> MTADELVFFVNGKKVVEKNADPETTLLAYLRRKLGLRGTKLGCGEGGCGACTVMLSKYDRLQDKIIHFSANACL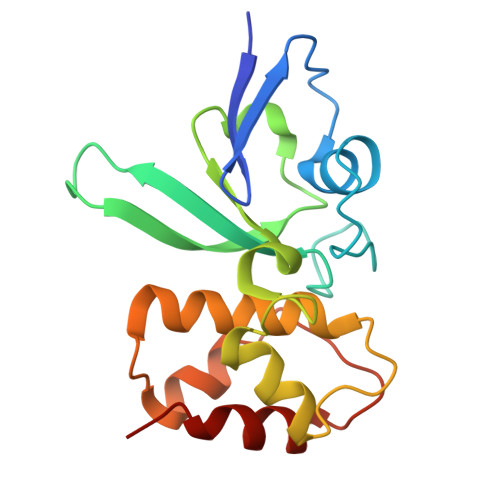APICTLHHVAVTTVEGIGSTKTRLHPVQERIAKSHGSQCGFCTPGIVMSMYTLLRNQPEPTVEEIEDAFQGNLCRCTGYRPILQGFRTFAK> GAQPTDPSTTDSELTMLVGTYT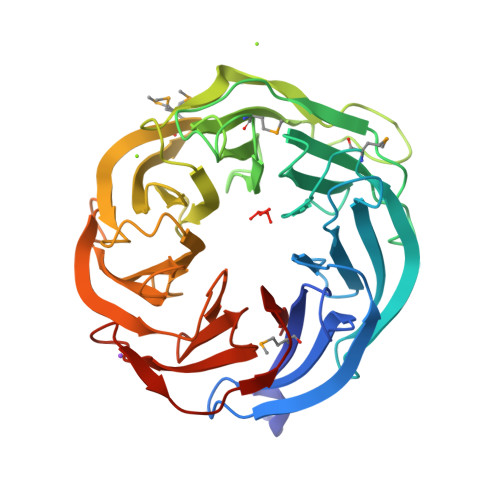SGNSKGIYTFRFNEETGESLPLSDAEVANPSYLIPSADGKFVYSVNEFSKDQAAVSAFAFDKEKGTLHLLNTQKTMGADPCYLTTNGKNIVTANYSGGSITVFPIGQDGALLPASDVIEFKGSGPDKERQTMPHLHCVRITPDGKYLLADDLGTDQIHKFNINPNANADNKEKFLTKGTPEAFKVAPGSGPRHLIFNSDGKFAYLINEIGGTVIAFRYADGMLDEIQTVAADTVNAQGSGDIHLSPDGKYLYASNRLKADGVAIFKVDETNGTLTKVGYQLTGIHPRNFIITPNGKYLLVACRDTNVIQIFERDQATGLLTDIKKDIKVDKPVCLKFVD>[3x]QGAVRKATAAEIAALPRQKV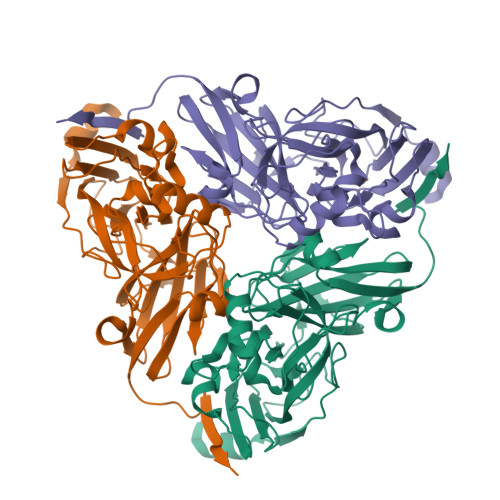ELVDPPFVHAHSQVAEGGPKVVEFTMVIEEKKIVIDDAGTEVHAMAFNGTVPGPLMVVHQDDYLELTLINPETNTLMHNIDFHAATGALGGGGLTEINPGEKTILRFKATKPGVFVYHCAPPGMVPWAVVSGMNGAIMVLPREGLHDGKGKALTYDKIYYVGEQDFYVPRDENGKYKKYEAPGDAYEDTVKVMRTLTPTHVVFNGAVGALTGDKAMTAAVGEKVLIVHSQANRDTRPHLIGGHGDYVWATGKFNTPPDVDQETWFIPGGAAGAAFYTFQQPGIYAYVNHNLIEAFELGAAAHFKVTGEWNDDLMTSVLAPSGT(2~{S})-3-azanyl-2-[[(1~{R})-5-[2-[4-[[2-(hydroxymethyl)imidazol-1-yl]methyl]phenyl]ethynyl]-2,3-dihydro-1~{H}-inden-1-yl]amino]-3-methyl-~{N}-oxidanyl-butanamide 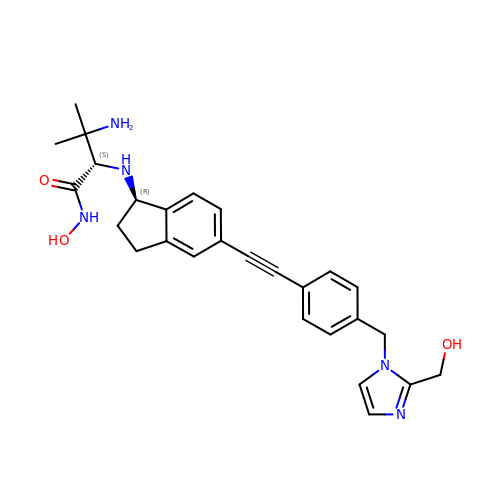| C27 H31 N5 O3 | HMFUASPGNDZNJF-ILBGXUMGSA-N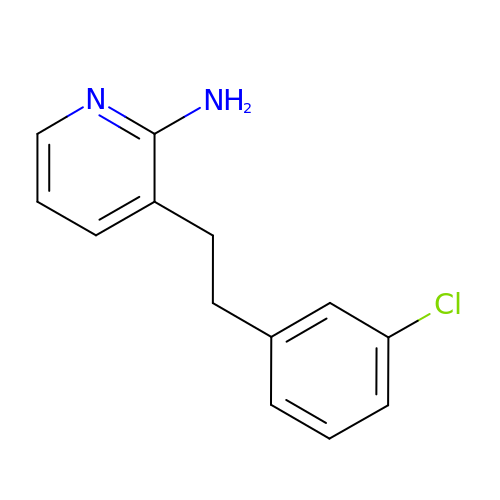3-[2-(3-chlorophenyl)ethyl]pyridin-2-amine | C13 H13 Cl N2 | XJCJGDOLNLEZIY-UHFFFAOYSA-N> PISPIETVPVKLKPGMDGPKVKQWPLTEEKIKALVEICTEMEKEGKISKIGPENPYNTPVFAIKKKDSTKWRKLVDFRELNKRTQDFWEVQLGIPHPAGLKKKKSVTVLDVGDAYFSVPLDEDFRKYTAFTIPSINNETPGIRYQYNVLPQGWKGSPAIFQSSMTKILEPFKKQNPDIVIYQYMDDLYVGSDLEIGQHRTKIEELRQHLLRWGLTTPDKKHQKEPPFLWMGYELHPDKWTVQPIVLPEKDSWTVNDIQKLVGKLNWASQIYPGIKVRQLSKLLRGTKALTEVIPLTEEAELELAENREILKEPVHGVYYDPSKDLIAEIQKQGQGQWTYQIYQEPFKNLKTGKYARMRGAHTNDVKQLTEAVQKITTESIVIWGKTPKFK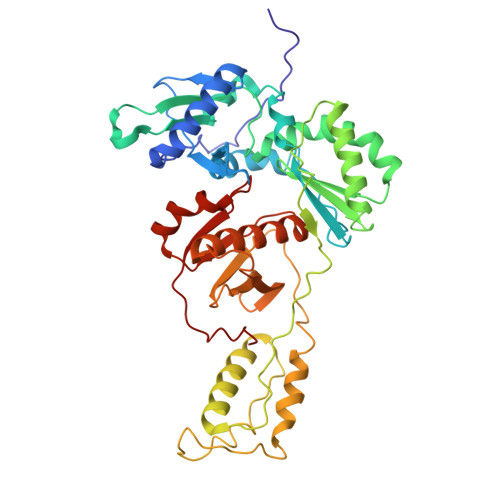LPIQKETWETWWTEYWQATWIPEWEFVNTPPLVKLWYQL>[2x]QEVEFDIPPQALGSALQEFGRQADIQVLYRPEEVRNKRSSAIKGKLEPNQAITELLRGTGASVDFQGNAITISVAEAADSSVDLGATMITSNQLGTITEDSGSYTPGTIATATRLVLTPRETPQSITVVTRQNMDDFGLNNIDDVMRHTPGITVSAYDTDRNNYYARGFSINNFQYDGIPSTARNVGYSAGNTLSDMAIYDRVEVLKGATGLLTGAGSLGATINLIRKKPTHEFKGHVELGAGSWDNYRS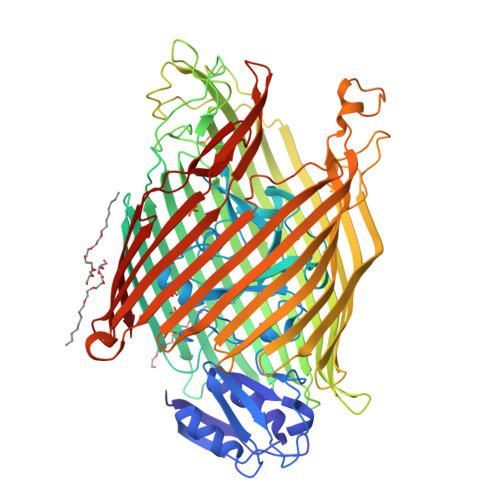ELDVSGPLTESGNVRGRAVAAYQDKHSFMDHYERKTSVYYGILEFDLNPDTMLTVGADYQDNDPKGSGWSGSFPLFDSQGNRNDVSRSFNNGAKWSSWEQYTRTVFANLEHNFANGWVGKVQLDHKINGYHAPLGAIMGDWPAPDNSAKIVAQKYTGETKSNSLDIYLTGPFQFLGREHELVVGTSASFSHWEGKSYWNLRNYDNTTDDFINWDGDIGKPDWGTPSQYIDDKTRQLGSYMTARFNVTDDLNLFLGGRVVDYRVTGLNPTIRESGRFIPYVGAVYDLNDTYSVYASYTDIFMPQDSWYRDSSNKLLEPDEGQNYEIGIKGEYLDGRLNTSLAYFEIHEENRAEEDALYNSKPTNPAITYAYKGIKAKTKGYEAEISGELAPGWQVQAGYTHKIIRDDSGKKVSTWEPQDQLSLYTSYKFKGALDKLTVGGGARWQGKSWQMVYNNPRSRWEKFSQEDYWLVDLMARYQITDKLSASVNVNNVFDKTYYTNIGFYTSASYGDPRNLMFSTRWDF> HKCDITLQEIIKDLNSLTEQKTLCTELTVTDIFAASKNTTEKETFCRAATVLRQFYSHHEKDTRCLGATAQQFHRHKQLIRFLKALDRNLWGLAGLNSCPVKEANQSTLENFLERLKTIMREKYSKCSS

Interleukin 4 (IL-4) is a pleiotropic cytokine that plays a major regulatory role in the immune system. Signal transduction of IL-4 is mediated by a sequential binding process, initiated first by binding of IL-4 to its high-affinity single membrane spanning receptor chain IL-4Rα. This intermediate ligand receptor complex then recruits one of two possible low-affinity receptor subunits, the common gamma chain (γc) or the IL-13Rα1 chain, into the functional hetero-trimeric complex to initiate signalling. The overall structure of IL-4 comprises the known four-helical bundle in up-up-down-down topology, which like the crystal packing is unaffected by these mutations.

We tested the interaction model proposed above by mutating Arg85 of IL-4 and the super-agonistic variants to alanine and measuring the residual binding affinity to IL-4Rα. If Arg85 is really involved in generating the additional stability/interaction, then, owing to cooperativity, mutation of this residue would have a greater effect in the super-agonistic variants (decrease in binding affinity) compared to wild-type IL-4. In contrast, the affinity of the IL-4 variant T13D-R85A is decreased 6.5-fold and its dissociation rate reflects IL-4 wild-type-like binding kinetics. Since the hallmark of the super-agonistic variants was a clearly decreased dissociation rate constant (relative koff (T13D or F82D) = 0.3 – 0.4 koff (IL-4wt)), this confirms the above mechanism by which Arg85 is involved in generating the higher binding affinity. To exclude the possibility that structural changes in addition to the removal of the Arg85 side chain play a role in the changes in binding stability, we determined the structures of the IL-4 variants R85A, T13D-R85A and F82D-R85A. No changes in the local structure around residues Thr/Asp13, Phe/Asp82 or Arg85 could be observed (data not shown).>MAHHHHHHMHKQTIKEVLENYKKFLHHDITVYGWVRAFRSNRFIALNDGSTINNLQIVVDFENFDENLIKNINTASSLKIVGEVVESQGAGQTVEIIAKKIIVLGDNFTEELQNTILQPKKHSLEKLREQAHLRFRTNLFGAVFRVRHAVSFAIHSFFNDRQFFYLNTPVITGADAEGAGEMFGVTNFDLDNIPRNEDGAIDYTQDFFGRKTNLTVSGQLEGETAAMGLGRIYTFGPTFRAENSNTTRHLAEFWMVEPEVAFNNLEDNIDLAEDFLKYVIQYVLDKCKDDLEFLDKRFAEEQKQKPEKERAKEGLIEKLENVVAKRFKRVSYTEAIDILLNSKENKKGKFVYPVEKWGADLQSEHERYLVEKHFECPVVLFDYPAEIKAFYMRLNEDNKTVAAMDVLFPG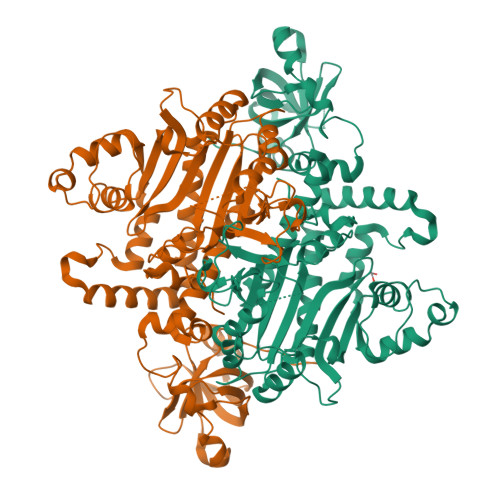IGEIIGGSQREERLDVLKKKMDDMHVDQEELWWYLDTRKFGSVPHSGFGLGLERLVLFVTGMTNIRDVIPFPRTPKNAEF[4x]>[4x]MSAFELKNLNDCLEKHLPPDELKEVKRIL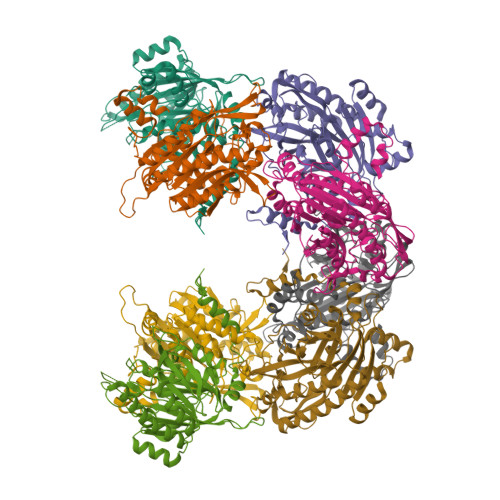YGVEEDQTLELPTSAKDIAEQNGFDIKGYRFTAREEQTRKRRIVRVGAIQNSIVIPTTAPIEKQREAIWNKVKTMIKAAAEAGCNIVCTQEAWTMPFAFCTREKFPWCEFAEEAENGPTTKMLAELAKAYNMVIIHSILERDMEHGETIWNTAVVISNSGRYLGKHRKNHIPRVGDFNESTYYMEGNTGHPVFETEFGKLAVNICYGRHHPQNWMMFGLNGAEIVFNPSATIGRLSEPLWSIEARNAAIANSYFTVPINRVGTEQFPNEYTSGDGNKAHKEFGPFYGSSYVAAPDGSRTPSLSRDKDGLLVVELDLNLCRQVKDFWGFRMTQRVPLYAESFKKASEHGFKPQIIKETQFPGDDDDKHHHHHHHHSG> MVLMELPKEMEEYFSMLQREIDKAYEIAKKARAQGKDPSLDVEIPQASDMAGRVESLVGPPGVAERIRELVKEYGKEIAALKIVDEIIDGKFGDLGSKEKYAEQAVRTALAILTEGVVSAPIEGIASVKIKRNTWSDNSEYLALYYAGPIRSSGGTAQALSVLVGDYVRRKLGLDRFKPSEKHIERMVEEVDLYHRTVSRLQYHPSPEEVRLAMRNIPIEITGEATDEVEVSHRDIPGVETNQLRGGAILVLAE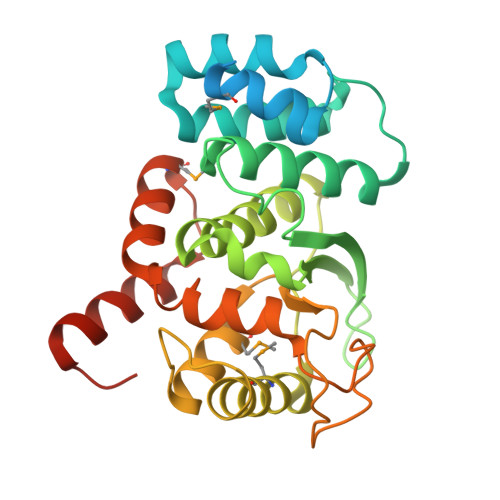GVLQKAKKLVKYIDKMGIEGWEWLKEFVEAKEKGEEIEEEGSAEST>GSTKDELTKIMDRASKIEQIQKLAKYAISALNYEDLPTAKDELTKALD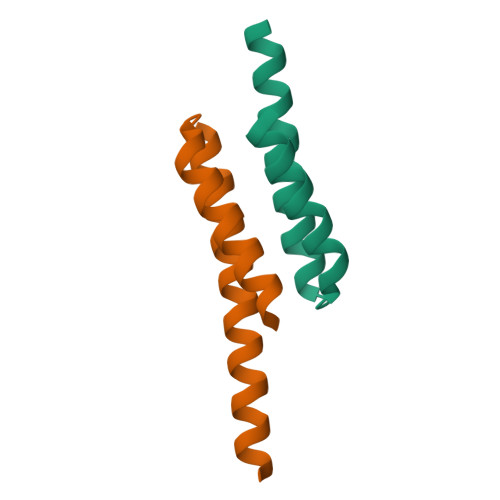LLNSI[6x]>[2x]MGSDKIHHHHHHVWEFYMPTDVFFGEKILEKRGNIIDLLGKRALVVTGKSS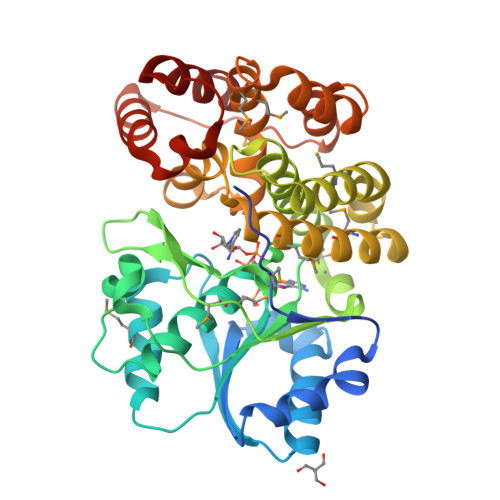SKKNGSLDDLKKLLDETEISYEIFDEVEENPSFDNVMKAVERYRNDSFDFVVGLGGGSPMDFAKAVAVLLKEKDLSVEDLYDREKVKHWLPVVEIPTTAGTGSEVTPYSILTDPEGNKRGCTLMFPVYAFLDPRYTYSMSDELTLSTGVDALSHAVEGYLSRKSTPPSDALAIEAMKIIHRNLPKAIEGNREARKKMFVASCLAGMVIAQTGTTLAHALGYPLTTEKGIKHGKATGMVLPFVMEVMKEEIPEKVDTVNHIFGGSLLKFLKELGLYEKVAVSSEELEKWVEKGSRAKHLKNTPGTFTPEKIRNIYREALGV4-[[4-azanyl-3-(4-cyclohexylpiperazin-1-yl)-9,10-bis(oxidanylidene)anthracen-1-yl]amino]benzoic acid | C31 H32 N4 O4 | 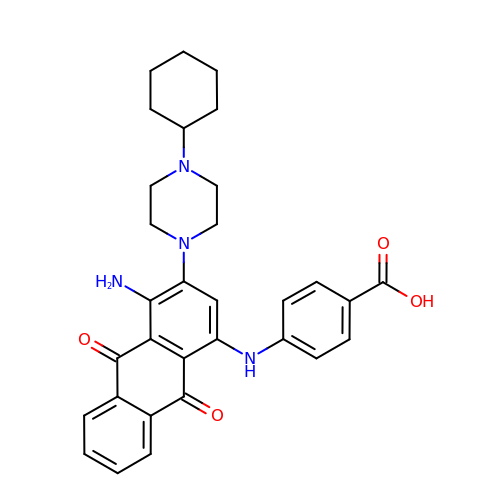YLGUWQFLCMWHDK-UHFFFAOYSA-N2,3,14,20,22-PENTAHYDROXYCHOLEST-7-EN-6-ONE | C27 H44 O6 | 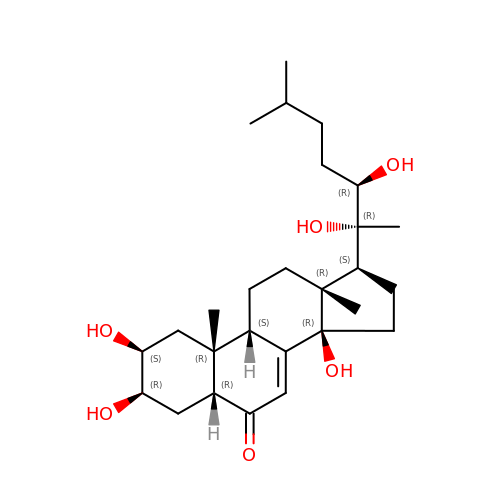PJYYBCXMCWDUAZ-JJJZTNILSA-N> MTTTMKISIEFLEPFRMTKWQESTRRNKNNKEFVRGQAFARWHRNKKDNTKGRPYITGTLLRSAVIRSAENLLTLSDGKISEKTCCPGKFDTEDKDRLLQLRQRSTLRWTDKNPCPDNAETYCPFCELLGRSGNDGKKAEKKDWRFRIHFGNLSLPGKPDFDGPKAIGSQRVLNRVDFKSGKAHDFFKAYEVDHTRFPRFEGEITIDNKVSAEARKLLCDSLKFTDRLCGALCVIRFDEYTPAADSGKQTENVQAEPNANLAEKTAEQIISILDDNKKTEYTRLLADAIRSLRRSSKLVAGLPKDHDGKDDHYLWDIGKKKKDENSVTIRQILTTSADTKELKNAGKWREFCEKLGEALYLKSKDMSGGLKITRRILGDAEFHGKPDRLEKSRSVSIGSVLKETVVCGELVAKTPFFFGAIDEDAKQTDLQVLLTPDNKYRLPRSAVRGILRRDLQTYFDSPCNAELGGRPCMCKTCRIMRGITVMDARSEYNAPPEIRHRTRINPFTGTVAEGALFNMEVAPEGIVFPFQLRYRGSEDGLPDALKTVLKWWAEGQAFMSGAASTGKGRFRMENAKYETLDLSDENQRNDYLKNWGWRDEKGLEELKKRLNSGLPEPGNYRDPKWHEINVSIEMASPFINGDPIRAAVDKRGTDVVTFVKYKAEGEEAKPVCAYKAESFRGVIRSAVARIHMEDGVPLTELTHSDCECLLCQIFGSEYEAGKIRFEDLVFESDPEPVTFDHVAIDRFTGGAADKKKFDDSPLPGSPARPLMLKGSFWIRRDVLEDEEYCKALGKALADVNNGLYPLGGKSAIGYGQVKSLGIKGDDKRISRLMNPAFDETDVAVPEKPKTDAEVRIEAEKVYYPHYFVEPHKKVEREEKPCGHQKFHE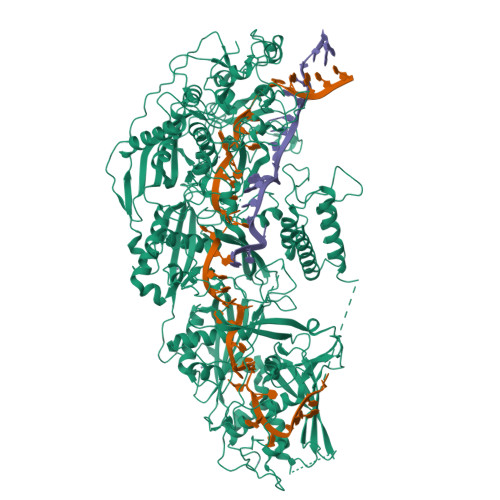GRLTGKIRCKLITKTPLIVPDTSNDDFFRPADKEARKEKDEYHKSYAFFRLHKQIMIPGSELRGMVSSVYETVTNSCFRIFDETKRLSWRMDADHQNVLQDFLPGRVTADGKHIQKFSETARVPFYDKTQKHFDILDEQEIAGEKPVRMWVKRFIKRLSLVDPAKHPQKKQDNKWKRRKEGIATFIEQKNGSYYFNVVTNNGCTSFHLWHKPDNFDQEKLEGIQNGEKLDCWVRDSRYQKAFQEIPENDPDGWECKEGYLHVVGPSKVEFSDKKGDVINNFQGTLPSVPNDWKTIRTNDFKNRKRKNEPVFCCEDDKGNYYTMAKYCETFFFDLKENEEYEIPEKARIKYKELLRVYNNNPQAVPESVFQSRVARENVEKLKSGDLVYFKHNEKYVEDIVPVRISRTVDDRMIGKRMSADLRPCHGDWVEDGDLSALNAYPEKRLLLRHPKGLCPACRLFGTGSYKGRVRFGFASLENDPEWLIPGKNPGDPFHGGPVMLSLLERPRPTWSIPGSDNKFKVPGRKFYVHHHAWKTIKDGNHPTTGKAIEQSPNNRTVEALAGGNSFSFEIAFENLKEWELGLLIHSLQLEKGLAHKLGMAKSMGFGSVEIDVESVRLRKDWKQWRNGNSEIPNWLGKGFAKLKEWFRDELDFIENLKKLLWFPEGDQAPRVCYPMLRKKDDPNGNSGYEELKDGEFKKEDRQKKLTTPWTPWA> GEFLATTLERIEKNFVITDPRLPDNPIIFASDSFLQLTEYSREEILGRNCRFLQGPETDRATVRKIRDAIDNQTEVTVQL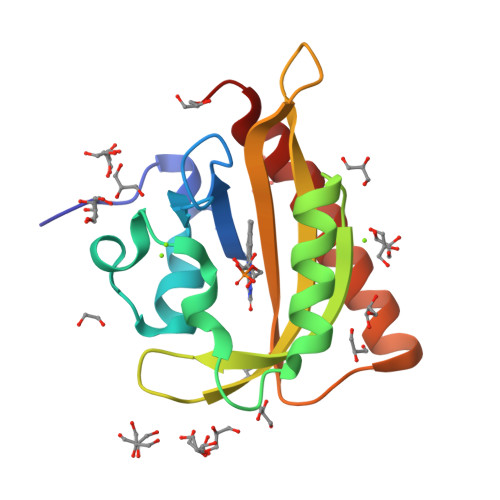INYTKSGKKFWNLFHLQPMRDQKGDVQYFIGVLLDGTEHVRDAAEREGVMLIKKTAENIDEAAKEL> AAAAAAAAA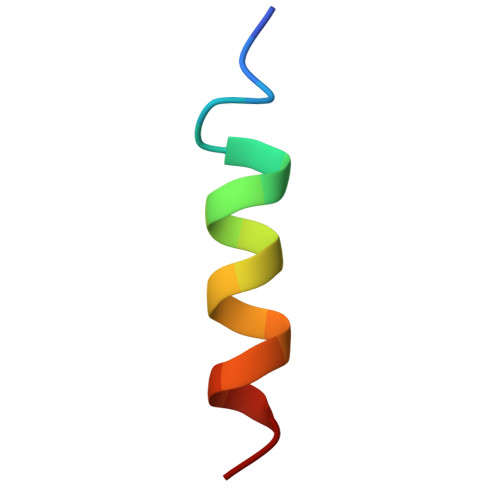AAAAAAAAAA>MSQVTEQSVRFQTALASIKLIQASAVLDLTEDDFDFLTSNKVWIATDRSRARRCVEACVYGTLDFVGYPRFPAPVEFIAAVIAYYVHPVNIQTACLIMEGAEFTENIINGVERPVKAAELFAFTLRVRAGNTDVLTDAEENVRQKLRAEGVM[4x];> MEQLTKNQRKKRDEIEAGKSYCSRRFGGATCDDKSAQIYARFDKNDWRIQPAEFYRFHDAEVNTFGYF;> MSNVQTSAEREIVDLSHLAFDCGMLGRLKTVSWTPVIAGDSFELDAVGALRLSPLRRGLAIDSKVDFFTFYIPHRHVYGDQWIQFMRDGVNAQPLPSVTCNRYPDHAGYVGTIVPANNRIPKFLHQSYLNIYNNYFRAPWMPERTEANPSNLNEDDARYGFRCCHLKNIWSAPLPPETKLAEEMGIESNSIDIMGLQAAYAQLHTEQERTYFMQRYRDVISSFGGSTSYDADNRPLLVMHTDFWASGYDVDGTDQSSLGQFSGRVQQTFKHSVPRFFVPEHGVMMTLALIRFPPISPLEHHYLAGKSQLTYTDLAGDPALIGNLPPREISYRDLFRDGRSGIKIKVAESIWYRTHPDYVNFKYHDLHGFPFLDDAPGTSTGDNLQEAILVRHQDYDACFQSQQLLQWNKQARYNVSVYRHMPTVRDSIMTS;> MYQNFVTKHDTAIQTSRFSVTGNVIPAAPTGNIPVINGGSITAERAVVNLYANMNVSTSSDGSFIVAMK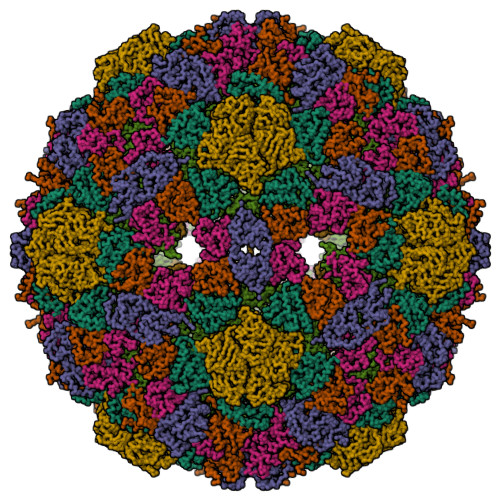VDTSPTDPNCVISAGVNLSFAGTSYPIVGIVRFESASEQPTSIAGSEVEHYPIEMSVGSGGVCSARDCATVDIHPRTSGNNVFVGVICSSAKWTSGRVIGTIATTQVIHEYQVLQPLK>XLAAALC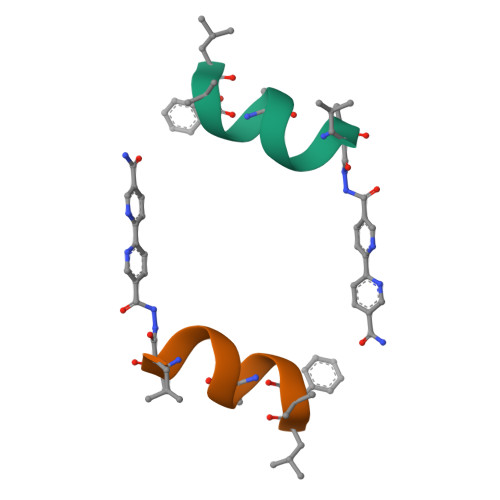QALX[2x]FimH is an adhesin positioned on the fimbrial tip which binds to mannosylated proteins on the urinary tract epithelium via its lectin domain (FimHLD). FimH is composed of two domains, an N-terminal lectin binding domain (FimHLD) responsible for binding to the terminal mannose moiety on epithelial glycoproteins, and a C-terminal pilin domain (FimHPD). FimHLD transitions between two endpoint conformations: a ‘closed’ conformation with a high affinity for mannosylated proteins, and an ‘open’ conformation with a relatively compressed structure, a wide mannose binding pocket, that binds to mannosylated proteins with low affinity. Conformation and ligand-binding properties of FimHLD are under the allosteric control of FimHPD, which itself exhibits only minor structural changes upon ligand binding.

Among all conformationally stabilized FimH-DSG mutants, FimH-DSG TM was of most interest as it harbors the two Glycine loop mutations G15A and G16A designed to conformationally lock the mannose binding site in the ‘open’ state. To verify the conformation of FimH-DSG TM, the crystal structure of a FimH-DSG TM protein containing three glycosylation site mutations (N7S, N70S, and N228Q) was solved by X-ray crystallography at 1.9 Å resolution. There are four molecules of FimH-DSG TM in one asymmetric unit which share high similarity, therefore, structural analysis was done with protomer A. Introduction of the glycosylation site mutations did not appear to alter either the local or global conformations of the FimHLD and FimHPD. Comparison of the structure to previously determined structures of FimHLD confirmed that FimH-DSG TM lectin domain adopts a compressed structure with an open mannose-binding pocket. Clear electron density was obtained for the Glycine loop, wherein the G15A G16A mutations were introduced which induced a local change in the loop conformation. A15 projects towards the inside region of the clamp loop, providing rigidity, which causes the loop to widen at the end by ~1.2 Å (I13 Cα-S17 Cα) compared to the WT residue (G15), thus stabilizing the low affinity state. Additional rigidity is introduced by the G16A substitution, as it projects towards the bulk solvent. In comparison to previously published structures, the donor strand complemented FimHPD did not exhibit any conformational changes. The backbone of the exogeneous 7-residue Glycine-Serine linker that connects the FimH and FimG peptide could largely be resolved, and does not impact the conformation of the lectin or pilin domains in comparison to previously published structures. Analysis by mass spectrometry confirmed that FimH-DSG retained a single glycosylation site at N235 in the exploratory antigen initially characterized in this study.

>[4x]FACKTASGTAIPIGAASANVYVNLAPAVNVGQNLVVDLSTQIFCHNDYPETITDYVTLQRGSAYGGVLSSFSGTVKYSGSSYPFPTTSETPRVVYNSRTDKPWPVALYLTPVSSAGGVAIKAGSLIAVLILRQTNNYNSDDFQFVWNIYANNDVVVPTGGCDVSARDVTVTLPDYPGSVPIPLTVYCAKSQNLGYYLSGTTADAGNSIFTNTASFSPAQGVGVQLTRQGTIIPANNTVSLGAVGTSAVSLGLTANYARTGGQVTAGNVQSIIGVTFVYQGGSSGGGADVTITVNGKVVAKGGHHHHHHHH>SVDTMALWLGLRAVLVVAGLAVLLQLIRGWLSSKSYVFNREEIARLAKEHSGLDYEVAFSKIIVELRKKHPGHILQDEDLQWVFVNAGGWMGSMCLLHASLTEYVLLFGTAVDTGGHSGRYWAEISDTILSG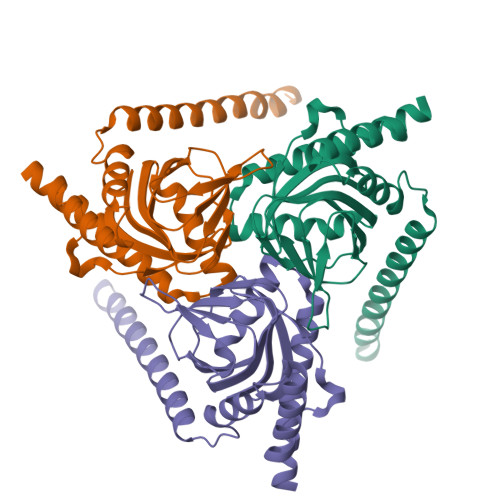TFRQWKEGTTKSEIFYPGDTIVHEVGEATSVQWSSGTWMVEYGRGFIPSTLAFALADTIFSTQDFLTLFYTVKVYSKALLLEASTHLSQLGFF[12x]> GAMGSSPNYDKWEMERTDITMKHKLGGGQYGEVYEGVWKKYSLTVAVKTLKEDTMEVEEFLKEAAVMKEIKHPNLVQLLGVCTREPPFYIITEFMTYGNLLDYLRECNRQEVNAVVLLYMATQISSAMEYLEKKNFIHRDLAARNCLVGENHLVKVADFGLSRLMTGDTYTAHAGAKFPIKWTAPESLAYNKFSIKSDVWAFGVLLWEIATYGMSPYPGIDLSQVYELLEKDYRMERPEGCPEKVYELMRACWQWNPSDRPSFAEIHQAFETMFQES

The pivotal driving force of the CML is the deregulation of the protein tyrosine kinase ABL1, which get constitutively expressed and activated due to genetic fusion of Abelson (ABL) gene with the chromosome 9 and 22 [t(9;22)(q34;q11)] of the break point cluster region (BCR) gene. The constitutive activation of the fused BCR-ABL kinase leads to the growth factors-independent proliferation and stimulate the downstream mediators such as STAT5, CRKL and ERK to remain the CML cells constitutive growth and survival. The first BCR-ABL inhibitor, Imatinib (Gleevec), as the seminal target therapy for the CML has achieved great clinical success and several other ABL inhibitors such as Nilotinib, Dasatinib, Bosutinib and Ponatinib have been developed to be used as the second line therapy to overcome a variety of the drug resistances induced by either various of point mutations or the chronic drug treatment induced BCR-ABL gene amplification. Here we report a novel type II BCR-ABL kinase /PDGFR dual kinase inhibitor, CHMFL-074, which exhibits high selectivity among the kinome and high potencies against both the native and a variety of clinically important mutants of BCR-ABL kinases both in vitro and in vivo.

The results demonstrated that CHMFL-074 adopted a typical type II binding mode (DFG-out conformation) to ABL1, which was represented by two canonical hydrogen bonds formed between the Glu286 located in the c-Helix and Asp381 located in the DFG motif with the amide bond (NHC=O) in the drug. However, superimposition of CHMFL-074 with Imatinib revealed a distinct hinge binding. CHMFL-074 used oxygen atom of carbonyl group connecting the terminal pyridine and piperidine ring to form the hinge binding hydrogen bonds with Met318, while Imatinib used the terminal pyridine ring's N atom to form this hinge binding. In addition, Imatinib formed an extra hydrogen bond between the aminopyrimidine's NH in the drug with the gatekeeper residue Thr315. However, CHMFL-074 used O-linked piperidine ring to replace this aminopyrimidine ring and abolished this hydrogen bond. The relatively rare binding mode of CHMFL-074, which uses carbonyl oxygen as the hinge binding, also highlights the new features of this type II compound. Further confirmation with Invitrogen Z'LYTE biochemical assay (activity-based assay) revealed an IC50 of 25 nM against ABL1 kinase. In addition, it also potently inhibited ABL1's mutants such as E255K, F317L, F317I, M351T, Q252H, Y253F but weakly inhibited H396P and almost lost the activity against the gatekeeper mutation T315I.> HPICEVSKVASHLEVNCDKRQLTALPPDLPKDTTILHLSENLLYTFSLATLMPYTRLTQLNLDRCELTKLQVDGTLPVLGTLDLSHNQLQSLPLLGQTLPALTVLDVSFNRLTSLPLGALRGLGELQ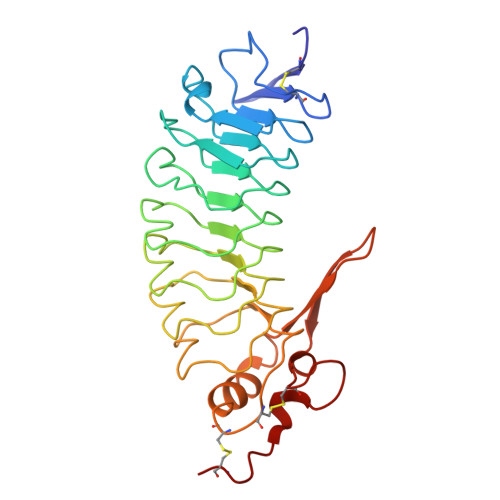ELYLKGNELKTLPPGLLTPTPKLEKLSLANNQLTELPAGLLNGLENLDTLLLQENSLYTIPKGFFGSHLLPFAFLHGNPWLCNCEILYFRRWLQDNAENVYVWKQGVDVKAMTSNVASVQCDNSDKFPVYKYPGKGCP>TIPDAMIVIDGHGIIQLFSTAAERLFGWSELEAIGQNVNILMPEPDRSRHDSYISRYRTTSDPHIIGIGRIVTGKRRDGTTFPMHLSIGEMQSGGEPYFTGFVRDLTEH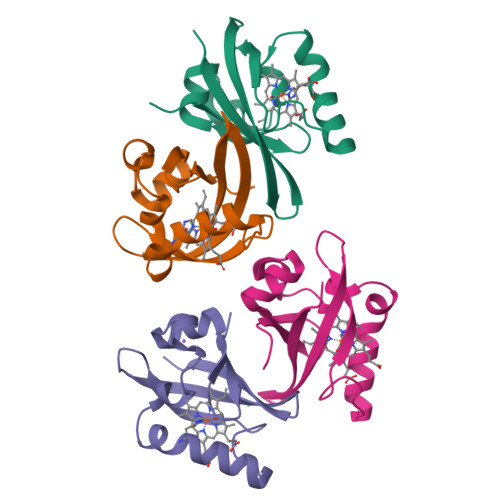QQTQARLQEL[4x]> HHHHHHMPSRTALSPGVLSPTRPVPNWIARPEYVGKPAAQEGSEPWVQTPEVIEKMRVAGRIAAGALAEAGKAVAPGVTTDELDRIAHEYLVDNGAYPSTLGYKGFPKSCCTSLNE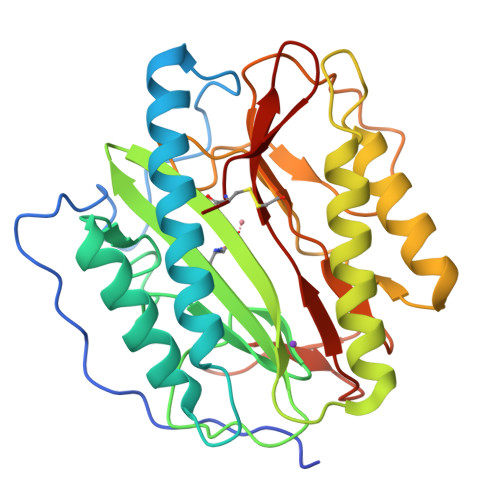VICHGIPDSTVITDGDIVNIDVTAYIGGVHGDTNATFPAGDVADEHRLLVDRTREATMRAINTVKPGRALSVIGRVIESYANRFGYNVVRDFTGHGIGTTFHNGLVVLHYDQPAVETIMQPGMTFTIEPMINLGALDYEIWDDGWTVVTKDRKWTAQFEHTLLVTDTGVEILTCL> GAMTFTRYSRLRVIAEIRHGDIFHSANIVSSIEFDRDDELFATAGVSRCIKVFDFSSVVNEPADMQCPIVEMSTRSKLSCLSWNKHEKNHIASSDYEGIVTVWDVTTRQSLMEYEEHEKRAWSVDFSRTEPSMLVSGSDDCKVKVWCTRQEASVINIDMKANICCVKYNPGSSNYIAVGSADHHIHYYDLRNISQPLHVFSGHKKAVSYVKFLSNNELASASTDSTLRLWDVKDNLPVRTFRGHTNEKNFVGLTVNSEYLACGSETNEVYVYHKEITRPVTSHRFGSPDMDDAEEEAGSYFISAVCWKSDSPTMLTANSQGTIKVLVLAA;> XEDQMVPSITY

The COP1 E3 ubiquitin ligase is a central signaling hub that integrates inputs from plant light‐sensing photoreceptors. COP1 contains an N‐terminal zinc finger, a central coiled‐coil, and a C‐terminal WD40 domain, which is essential for proper COP1 function (Deng et al, 1992; McNellis et al, 1994). COP1 regulates gene expression and plays a central role as a repressor of photomorphogenesis by directly modulating the stability of transcription factors that control the expression of light‐regulated genes.

Indeed, CRY1 and CRY2 also contain potential VP peptide motifs within their CCT domains, but their function in blue‐light signaling has not been established. Next, we obtained crystal structures for the different peptides bound to COP1 (1.3–2.0 Å resolution, see Tables EV1 and EV2, and EV4) to compare their peptide binding modes. We found that all peptides bind in a similar configuration with the VP forming the center of the binding site (r.m.s.d. between the different peptides range from ~ 0.3 to 1.5 Å, comparing 5 or 6 corresponding Cα atoms). Chemically diverse amino acids (Tyr/Arg/Gln) map to the −3 and −2 position and often deeply insert into the COP1 binding cleft, acting as anchor residues. This suggests that the COP1 WD40 domain has high structural plasticity, being able to accommodate sequence‐divergent VP‐containing peptides. As for UVR8, COP1Lys422Ala showed increased binding affinity for some peptides such as those representing the COL3287–294 and CO366–373 VP motifs, while it reduced binding to others, such as to CRY1544–552 and CRY2527–535. These observations may be rationalized by an enlarged VP‐binding pocket in the COP1Lys422Ala mutant, increasing accessibility for the COL3Phe288 anchor residue, and potentially abolishing interactions with CRY1Asp545. Independent of this, it is interesting to note that the hy4‐9 mutant, which replaces the proline in the CRY1 VP peptide motif with leucine, does not show inhibition of hypocotyl elongation under blue light (Ahmad et al, 1995). Similarly, the VP motif in the CCT domain of cryptochromes may become exposed and available for interaction upon blue‐light activation of the photoreceptor (Müller & Bouly, 2015; Wang et al, 2018).>MYSTAVLLNKISPTRDGQTMTLADLQYLSFSELRKIFDDQLSWGEARHLYHETIEQKKNNRLLEARIFTRANPQLSGAIRLGIERDSVSRSYDEMFGARSSSFVKPGSVASMFSPAGYLTELYREAKDLHFSSSAYHLDNRRPDLADLTLSQSNMDTEISTLTLSNELLLEHITRKTGGDSDALMESLSTYRQAIDTPYHQPYETIRQVIMTHDSTLSALSRNPEVMGQAEGASLLAILANISPELYNILTEEITEKNADALFAQNFSENITPENFASQSWIAKYYGLELSEVQKYLGMLQNGYSDSTSAYVDNISTGLVVNNESKLEAYKITRVKTDDYDKNINYFDLMYEGNNQFFIRANFKVSREFGATLRKNAGPSGIVGSLSGPLIANTNFKSNYLSNISDSEYKNGVKIYAYRYTSSTSATNQGGGIFTFESYPLTIFALKLNKAIRLCLTSGLSPNELQTIVRSDNAQGIINDSVLTKVFYTLFYSHRYALSFDDAQVLNGSVINQYADDDSVSHFNRLFNTPPLKGKIFEADGNTVSIDPDEEQSTFARSALMRGLGVNSGELYQLGKLAGVLDAQNTITLSVFVISSLYRLTLLARVHQLTVNELCMLYGLSPFNGKTTASLSSGELPRLVIWLYQVTQWLTEAEITTEAIWLLCTPEFSGNISPEISNLLNNLRPSISEDMAQSHNRELQAEILAPFIAATLHLASPDMARYILLWTDNLRPGGLDIAGFMTLVLKESLNANETTQLVQFCHVMAQLSLSVQTLRLSEAELSVLVISGFAVLGAKNQPAGQHNIDTLFSLYRFHQWINGLGNPGSDTLDMLRQQTLTADRLASVMGLDISMVTQAMVSAGVNQLQCWQDINTVLQWIDVASALHTMPSVIRTLVNIRYVTALNKAESNLPSWDEWQTLAENMEAGLSTQQAQTLADYTAERLSSVLCNWFLANIQPEGVSLHSRDDLYSYFLIDNQVSSAIKTTRLAEAIAGIQLYINRALNRIEPNARADVSTRQFFTDWTVNNRYSTWGGVSRLVYYPENYIDPTQRIGQTRMMDELLENISQSKLSRDTVEDAFKTYLTRFETVADLKVVSAYHDNVNSNTGLTWFVGQTRENLPEYYWRNVDISRMQAGELAANAWKEWTKIDTAVNPYKDAIRPVIFRERLHLIWVEKEEVAKNGTYWKTPVETYDRFTLKLAFLRHDGSWSAPWSYDITTQVEAVTDKKPDTERLALAASGFQGEDTLLVFVYKTGKSYSDFGGSNKNVAGMTIYGDGSFKKMENTALSRYSQLKNTFDIIHTQGNDLVRKASYRFAQDFEVPASLNMGSAIGDDSLTVMENGNIPQITSKYSSDNLAITLHNAAFTVRYDGSGNVIRNKQISAMKLTGVDGKSQYGNAFIIANTVKHYGGYSDLGGPITVYNKTKNYIASVQGHLMNADYTRRLILTPVENNYYARLFEFPFSPNTILNTVFTVGSNKTSDFKKCSYAVDGNNSQGFQIFSSYQSSGWLDIDTGINNTDIKITVMAGSKTHTFTASDHIASLPANSFDAMPYTFKPLEIDASSLAFTNNIAPLDIVFETKAKDGRVLGKIKQTLSVKRVNYNPEDILFLRETHSGAQYMQLGVYRIRLNTLLASQLVSRANTGIDTILTMETQRLPEPPLGEGFFANFVLPKYDPAEHGDERWFKIHIGNVGGNTGRQPYYSGMLSDTSETSMTLFVPYAEGYYMHEGVRLGVGYQKITYDNTWESAFFYFDETKQQFVLINDADHDSGMTQQGIVKNIKKYKGFLNVSIATGYSAPMDFNSASALYYWELFYYTPMMCFQRLLQEKQFDEATQWINYVYNPAGYIVNGEIAPWIWNCRPLEETTSWNANPLDAIDPDAVAQNDPMHYKIATFMRLLDQLILRGDMAYRELTRDALNEAKMWYVRTLELLGDEPEDYGSQQWAAPSLSGAASQTVQAAYQQDLTMLGRGGVSKNLRTANSLVGLFLPEYNPALTDYWQTLRLRLFNLRHNLSIDGQPLSLAIYAEPTDPKALLTSMVQASQGGSAVLPGTLSLYRFPVMLERTRNLVAQLTQFGTSLLSMAEHDDADELTTLLLQQGMELATQSIRIQQRTVDEVDADIAVLAESRRSAQNRLEKYQQLYDEDINHGEQRAMSLLDAAAGQSLAGQVLSIAEGVADLVPNVFGLACGG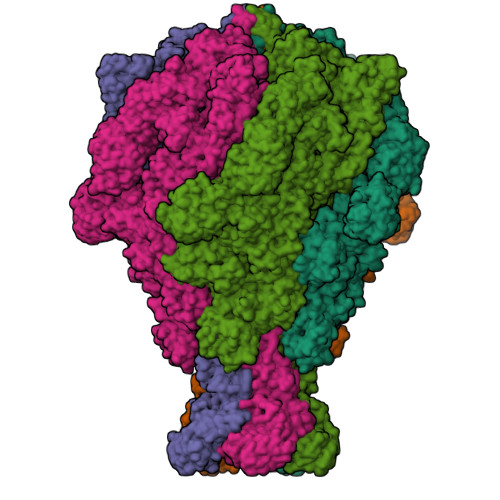SRWGAALRASASVMSLSATASQYSADKISRSEAYRRRRQEWEIQRDNADGEVKQMDAQLESLKIRREAAQMQVEYQETQQAHTQAQLELLQRKFTNKALYSWMRGKLSAIYYQFFDLTQSFCLMAQEALRRELTDNGVTFIRGGAWNGTTAGLMAGETLLLNLAEMEKVWLERDERALEVTRTVSLAQFYQALSSDNFNLTEKLTQFLREGKGNVGASGNELKLSNRQIEASVRLSDLKIFSDYPESLGNTRQLKQVSVTLPALVGPYEDIRAVLNYGGSIVMPRGCSAIALSHGVNDSGQFMLDFNDSRYLPFEGISVNDSGSLTLSFPDATDRQKALLESLSDIILHIRYTIR[5x]> GSHMVPDTPTRLVFSALGPTSLRVSWQEPRCERPLQGYSVEYQLLNGGELHRLNIPNPAQTSVVVEDLLPNHSYVFRV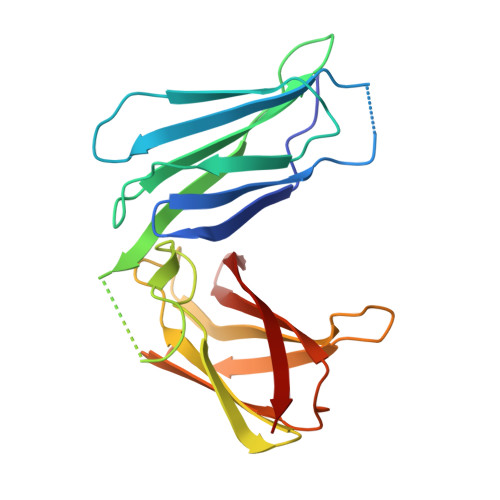RAQSQEGWGREREGVITIESQVHPQSPLCPLPGSAFTLSTPSAPGPLVFTALSPDSLQLSWERPRRPNGDIVGYLVTCEMAQGGGPATAFRVDGDSPESRLTVPGLSENVPYKFKVQARTTEGFGPEREGIITIES> MDAYSTRPLTLSHGSLEHVLLVPTASFFIASQLQEQFNKILPEPTEGFAADDEPTTPAELVGKFLGYVSSLVEPSKVGQFDQVLNLCLTEFENCYLEGNDIHALAAKLLQENDTTLVKTKELIKNYITARIMAKRPFDKKSNSALFRAVGEGNAQLVAIFGGQGNTDDYFEELRDLYQTYHVLVGDLIKFSAETLSELIRTTLDAEKVFTQGLNILEWLENPSNTPDKDYLLSIPISCPLIGVIQLAHYVVTAKLLGFTPGELRSYLKGATGHSQGLVTAVAIAETDSWESFFVSVRKAITVLFFIGVRCYEAYPNTSLPPSILEDSLENNEGVPSPMLSISNLTQEQVQDYVNKTNSHLPAGKQVEISLVNGAKNLVVSGPPQSLYGLNLTLRKAKAPSGLDQSRIPFSERKLKFSNRFLPVASPFHSHLLVPASDLINKDLVKNNVSFNAKDIQIPVYDTFDGSDLRVLSGSISERIVDCIIRLPVKWETTTQFKATHILDFGPGGASGLGVLTHRNKDGTGVRVIVAGTLDINPDDDYGFKQEIFDVTSNGLKKNPNWLEEYHPKLIKNKSGKIFVETKFSKLIGRPPLLVPGMTPCTVSPDFVAATTNAGYTIELAGGGYFSAAGMTAAIDSVVSQIEKGSTFGINLIYVNPFMLQWGIPLIKELRSKGYPIQFLTIGAGVPSLEVASEYIETLGLKYLGLKPGSIDAISQVINIAKAHPNFPIALQWTGGRGGGHHSFEDAHTPMLQMYSKIRRHPNIMLIFGSGFGSADDTYPYLTGEWSTKFDYPPMPFDGFLFGSRVMIAKEVKTSPDAKKCIAACTGVPDDKWEQTYKKPTGGIVTVRSEMGEPIHKIATRGVMLWKEFDETIFNLPKNKLVPTLEAKRDYIISRLNADFQKPWFATVNGQARDLATMTYEEVAKRLVELMFIRSTNSWFDVTWRTFTGDFLRRVEERFTKSKTLSLIQSYSLLDKPDEAIEKVFNAYPAAREQFLNAQDIDHFLSMCQNPMQKPVPFVPVLDRRFEIFFKKDSLWQSEHLEAVVDQDVQRTCILHGPVAAQFTKVIDEPIKSIMDGIHDGHIKKLLHQYYGDDESKIPAVEYFGGESPVDVQSQVDSSSVSEDSAVFKATSSTDEESWFKALAGSEINWRHASFLCSFITQDKMFVSNPIRKVFKPSQGMVVEISNGNTSSKTVVTLSEPVQGELKPTVILKLLKENIIQMEMIENRTMDGKPVSLPLLYNFNPDNGFAPISEVMEDRNQRIKEMYWKLWIDEPFNLDFDPRDVIKGKDFEITAKEVYDFTHAVGNNCEDFVSRPDRTMLAPMDFAIVVGWRAIIKAIFPNTVDGDLLKLVHLSNGYKMIPG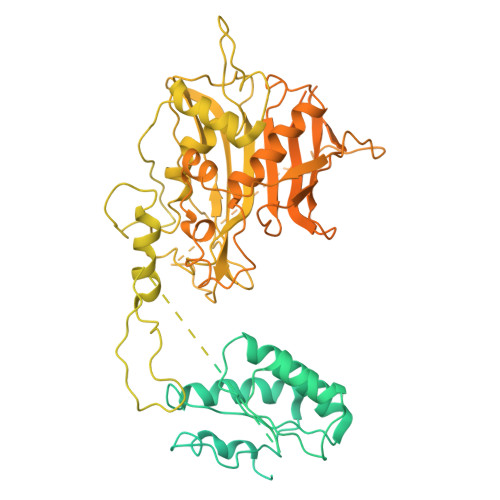AKPLQVGDVVSTTAVIESVVNQPTGKIVDVVGTLSRNGKPVMEVTSSFFYRGNYTDFENTFQKTVEPVYQMHIKTSKDIAVLRSKEWFQLDDEDFDLLNKTLTFETETEVTFKNANIFSSVKCFGPIKVELPTKETVEIGIVDYEAGASHGNPVVDFLKRNGSTLEQKVNLENPIPIAVLDSYTPSTNEPYARVSGDLNPIHVSRHFASYANLPGTITHGMFSSASVRALIENWAADSVSSRVRGYTCQFVDMVLPNTALKTSIQHVGMINGRKLIKFETRNEDDVVVLTGEAEIEQPVTTFVFTGQGSQEQGMGMDLYKTSKAAQDVWNRADNHFKDTYGFSILDIVINNPVNLTIHFGGEKGKRIRENYSAMIFETIVDGKLKTEKIFKEINEHSTSYTFRSEKGLLSATQFTQPALTLMEKAAFEDLKSKGLIPADATFAGHSLGEYAALASLADVMSIESLVEVVFYRGMTMQVAVPRDELGRSNYGMIAINPGRVAASFSQEALQYVVERVGKRTGWLVEIVNYNVENQQYVAAGDLRALDTVTNVLNFIKLQKIDIIELQKSLSLEEVEGHLFEIIDEASKKSAVKPRPLKLERGFACIPLVGISVPFHSTYLMNGVKPFKSFLKKNIIKENVKVARLAGKYIPNLTAKPFQVTKEYFQDVYDLTGSEPIKEIIDNWEKYEQSHHHHHH>SMSLSTRIAPHLPYLRRFARSVTG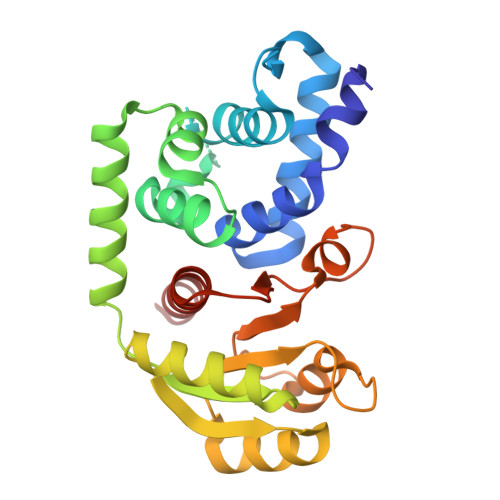SQSSGDAYVSAMLEALVADISIFPRASCDRIGTYWLFCHLFDQTTPNIPEPLPQFGLEQKTSAKLSYLTPRARQAFLLIAVEGFNEQEASEIMNLDARDFRKLLNQASIDISQQIATQVMIIEDEPLIAMDIEQMVESLGHQVVGIARTRKEAVVMYHQKKPRLILADIQLADNSSGIDAVNDILQNDRIPVIFITAFPERLLTGERPEPTFLVTKPFNPDMVKALISQALFFKENASKAA[2x]>KKHTGYVGLKNQGATCYMNSLLQTLFFTNQLRKAVYMMPTEGDDSSKSVPLALQRVFYELQHSDKPVGTKKLTKSFGWETLDSFMQHDVQELCRVLLDNVENKMKGTCVEGTIPKLFRGKMVSYIQCKEVDYRSDRREDYYDIQLSIKGKKNIFESFVDYVAVEQLDGDNKYDAGEHGLQEAEKGVKFLTLPPVLHLQLMRFMYDPQTDQNIKINDRFEFPEQLPLDEFLQKTDPKDPANYILHAVLVHSGDNHGGHYVVYLNPKGDGKWCKFDDDVVSRCTKEEAIEHNYGGHDDDLSVRHCTNAYMLVYIRESKLSEVLQAVTDHDIPQQLVERLQEEKRIEAQKRKE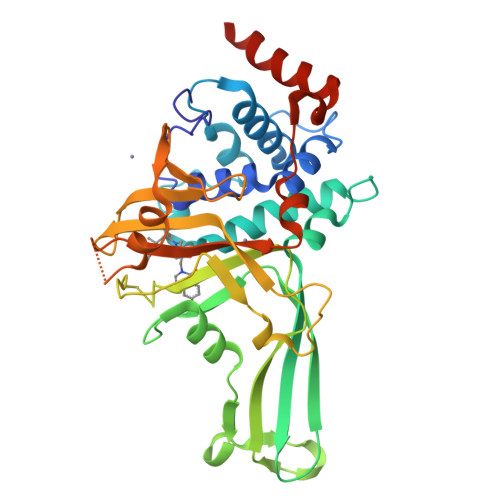RQE[2x]> MKNTTLYTYRDYFVIRGGKPLTGKVKISGAKNAALPIMFATILTEEPCTITNVPDLLDVRNTLLLLRELGAELEFLNNTVFINPSINSFITNQEIIRRMRASVLSLGPLLGRFGRAVVGLPGGCSIGARPIDQHLKFFKEAGADVEVREGYVYVNLKEKRRVHFKFDLVTVTGTENALLYLASVPEESILENIALEPEVMDLIEVLKKMG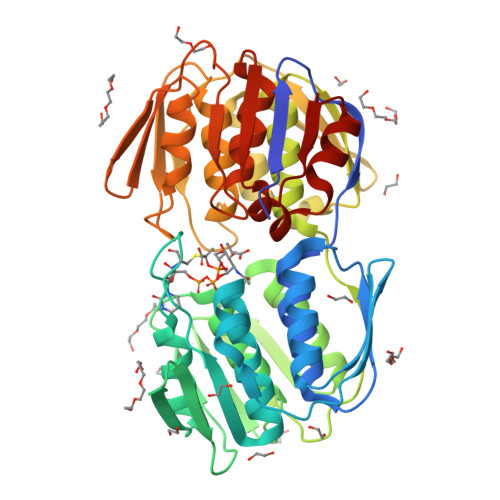AHVKVEGRSAYVKGSENLKGFTHSVIPDRIEAGTFMVGAVLTDGEILLENARINHLRAVVEKLKLIGGEVVEENGNLRVFRKESLRACDIETQVYPGFPTDMQAQFMALLSVAKGKSRIKENIFEHRFHHAQELNRLGANITVRGNTAYVEGVERLYGSEVYSTDLRASASLVLAGLVAQGETVVRDVYHLDRGYEKLEEKLKKLGADIERVSEL>GSGAVTAGAAPRILKHQVVRAELDRMLDGMRIGDPFPAEREIAEQFEVARETVRQALRELLIDGRVERRGRTTVVARPKIRQPLGMGSYTEAAKAQGLSAGRILVAWSDLTADEVLAGVLGVDVGAPVLQLERVLTTDGVRV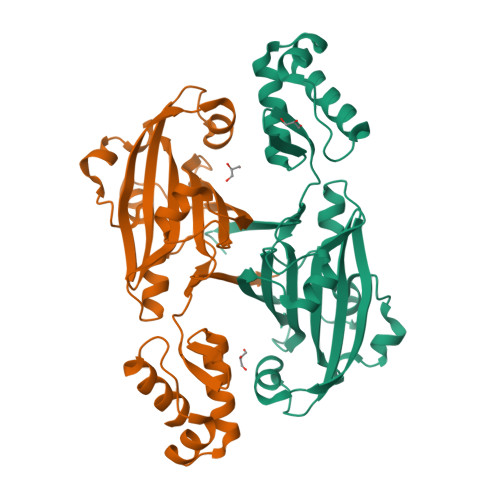GLETTKLPAQRYPGLRETFDHEASLYAEIRSRGIAFTRTVDTIDTALPDAREAALLGADARTPMFLLNRVSYDQDDVAIEQRRSLYRGDRMTFTAVMHAKNSAIVS[2x]>[4x]GSHMAYTLKVHYKYTVVMKTQPGLPYSQVRDMVSKKLELRLEHTKLSYRPRDSNELVPLSEDSMKDAWGQVKN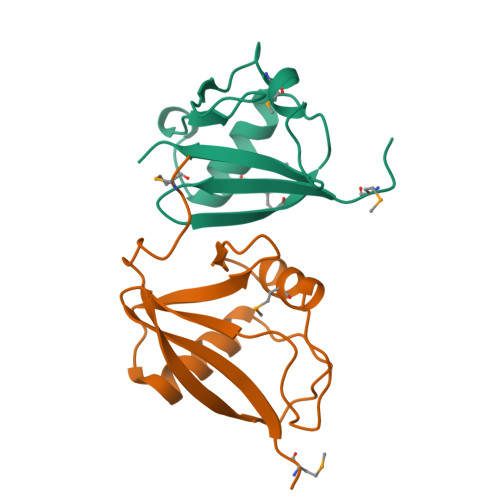YCLTLWCENT;>GSHMTNWLRVYYYEDTISTIKDIAVEEDLSSTPLLKDLLELTRREFQREDIALNYRDAEGDLVRLLSDEDVALMVRQARGLPSQKRLFPWKLHITQKDNYRVYNTMP[4x]>[3x]GPSQNAIKRFMTLFSGREDVFSIQY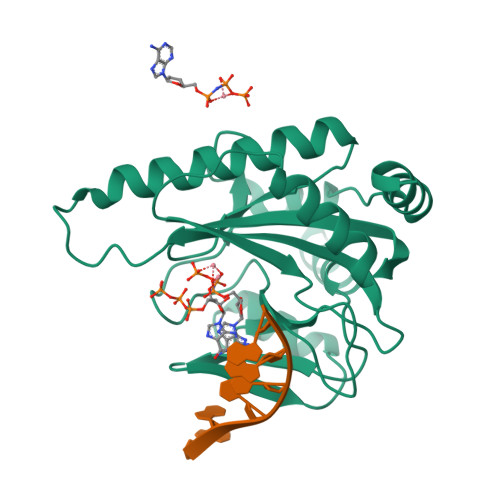EGGYRPIRRPLNFQDIKNHFSGKKTLGIYLLKKNDTVKFAAYDIDIKKHYLNREDKFVYEENSKKVAKRLSRELNLENITHYFEFTGNRGYHIWIFFDIPVSAYKIKYIMEKILDRIELEEGIDVEIFPKQTSLNGGLGNLIKVPLGVHKKTGKKCLFVDNDFNVIENQIEFLNNIKENKATEINKLFREIFNE> MVDGNYSVASNVMVPMRDGVRLAVDLYRPDADGPVPVLLVRNPYDKFDVFAWSTQSTNWLEFVRDGYAVVIQDTRGLFASEGEFVPHVDDEADAEDTLSWILEQAWCDGNVGMFGVSYLGVTQWQAAVSGVGGLKAIAPSMASADLYRAPWYGPGGALSVEALLGWSALIGRQLITSRSDARPEDAADFVQLAAILNDVAGAASVTPLAEQPLLGRLIPWVIDQVVDHPDNDESWQSISLFERLGGLATPALITAGWYDGFVGESLRTFVAVKDNADARLVVGPWSHSNLTGRNADRKFGIAATYPIQEATTMHKAFFDRHLRGETDALAGVPKVRLFVMGIDEWRDETDWPLPDTAYTPFYLGGSGAANTSTGGGTLSTSISGTESADTYLYDPADPVPSLGG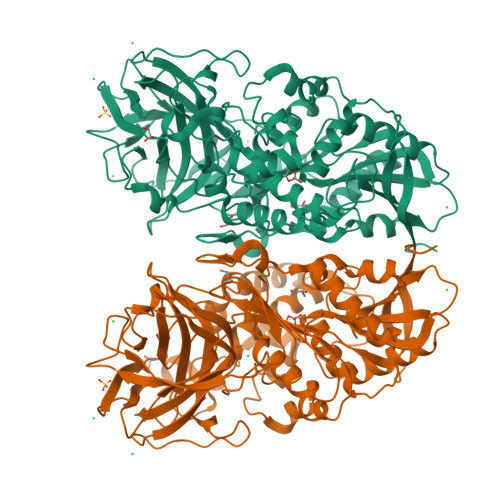TLLFHNGDNGPADQRPIHDRDDVLCYSTEVLTDPVEVTGTVSARLFVSSSAVDTDFTAKLVDVFPDGRAIALCDGIVRMRYRETLVNPTLIEAGEIYEVAIDMLATSNVFLPGHRIMVQVSSSNFPKYDRNSNTGGVIAREQLEEMCTAVNRIHRGPEHPSHIVLPIIKRKLAAALEHHHHHH(3S)-3-[(1R)-2-{[(4S)-6-ethyl-3,4-dihydrospiro[chromene-2,1'-cyclobutan]-4-yl]amino}-1-hydroxyethyl]-4-azabicyclo[10.3.1]hexadeca-1(16),12,14-trien-5-one 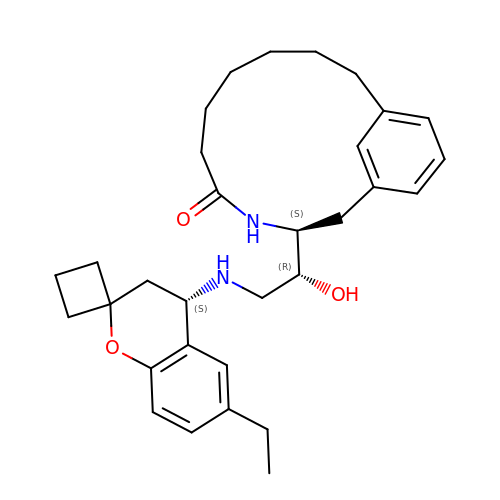| C31 H42 N2 O3 | NUISAGYICVEVAE-HZFUHODCSA-N> GPLGSFTSEKGVVEEWLSEFKTLPETSLPNYATNLKDKSSLVSSLYKVIQEPQSELLEPVCHQLFEFYRSGEEQLLQFTLQFLPELIWCYLAVSASRNVHSSGCIEALLLGVYNLEIVDKQGHTKVLSFTIPSLSKPSVYHEPSSIGSMALTESALSQHGLSKVVYSGPHPQREML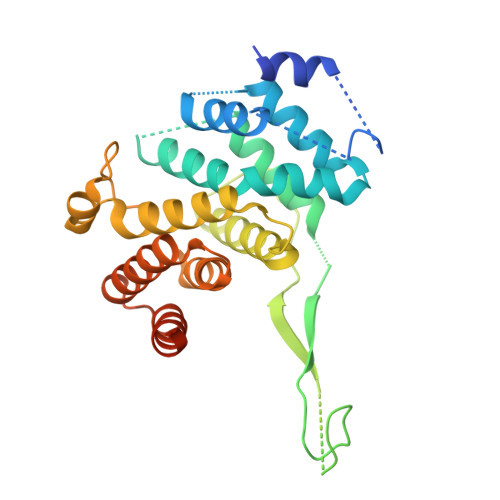TAQNRFEVLTFLLLCYNAALTYMPSVSLQSLCQICSRICVCGYPRQHVRKYKGISSRIPVSSGFMVQMLTGIYFAFYNGEWDLAQKALDDIIYRAQLELYPEPLLVANAIKASLPHGPMKSNKEGTRCIQVEITPT> MITMKDIIKEGHPTLRKVAEPVPLPPSEEDKRILQSLLDYVKMSQDPELAAKYGLRPGIGLAAPQINVSKRMIAVHVTDENGTLYSYALFNPKIVSHSVQQCYLTTGEGCLSVDRDVPGYVLRYARITVTGTTLDGEEVTLRLKGLPAIVFQHEIDHLNGIMFYDRINPADPFQVPDGAIP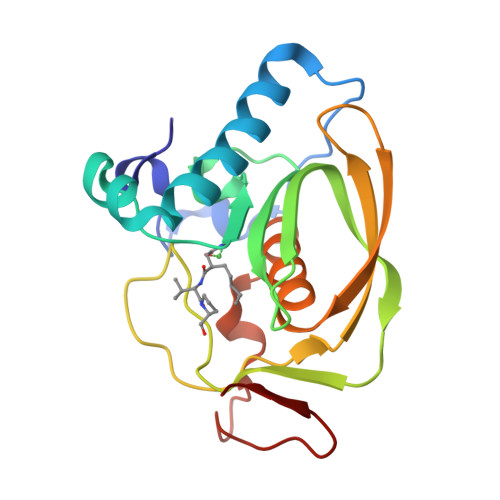IGR To gain insight into IniA-mediated drug resistance, we determined the structure of full-length IniA from Mycobacterium smegmatis (M. smegmatis), which shares 68% sequence identity with IniA from Mycobacterium tuberculosis (M. tuberculosis). IniA consists of an N-terminal GTPase domain and two HBs. Here, we determined structures of IniA, with and without bound GTP, and demonstrated that it mediates membrane fission in vitro. Our results suggested that IniA, like other BDLPs, has weak GTPase activity and nucleotide-dependent dimerization in solution, but tends to form nucleotide-independent homotypic interactions on the membrane and cuts the membrane.

We also determined the structure of nucleotide-free IniA at 3.2 Å resolution by molecular replacement using the GTP-bound structure as a search model. Overall, the apo state of IniA adopts a very similar fold as the GTP state, with a root-mean-square deviation of only 0.525 Å. An IniA dimer with antiparallel packing of HB2 was found in the asymmetric unit. However, we discovered no such interface but a HB2-stacking dimer in the crystal packing of our structures. Symmetric interactions of a D333α7–R351α7’ salt bridge and D337α7–H344α7’, E402α8–H348α7’ hydrogen bonds are observed between the antiparallel HB2s. When purified IniA triple-mutant D333K/D337K/E402K was incubated with liposomes, tethering of vesicles was not altered. However, when the HB2 was deleted, tethering could no longer be observed, suggesting a minor role of the HB2-stacking interface but a requirement of the HB2 in IniA self-assembly.

>[2x]MGVIVELIDHTSAIAAAKDRADLVERLRAAKARISDPQIRVVIAGQLKQGKSQLLNSLLNIPVARVGDDESTVLATVVSYGEQASARLVVARPDGAEPELIEIPPSEVTTDLRRAPQASGRQVLRVEVTAPSPLLKGGLAFVDTPGVGGHGQPHLSATLGLLPDADAMLMISDTSQEFTEPEMKFIRQALEICPVAAIVATKTDLYPHWRQIVDANIAHLQRAGLNVPVIPASSVLRSHAISLNDKELNEESNFPAIVKFLSEHVLSRQNDRIRDQIVDEIRSAAEHLLLAVESELSSFNDPGERERLTAELERRKQEAQDALQQTALWQQVLSDGIADLTADVDHDLRHRFRIIAAHTEKVIDGCDPTLHWAEIGAELEDAVATAVGDNFVWAYQRAEALAAEVARTFTEAGLDAVQMPQIDARDMGAGFGELNSLARLEAKPIKIGHKVVTGMRGSYGGVLMFGMLTSFAGLGMFNPLSLGAGFVLGRKAYKEDMENRMLRVRNEAKANVRKFVDDVAFVVGKESRDRLKGIQRQLRDHYREIANQTTRSLNESLQAAIAAAKVEEAERNTRVKELERQQNILKQVVDHAAKLAAALEHHHHHH6-benzyl-5-chloro[1,2,4]triazolo[1,5-a]pyrimidin-7(3H)-one | C12 H9 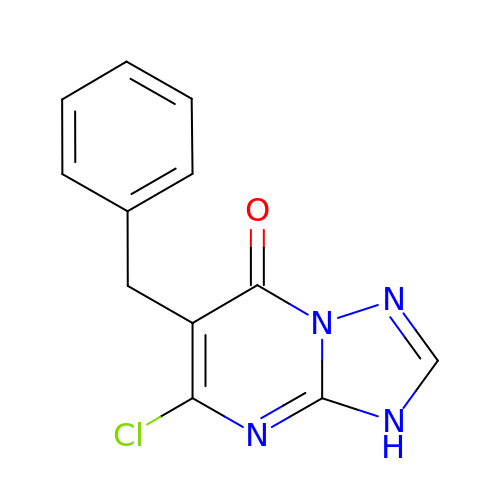Cl N4 O | MQEBPOLOTAZMKF-UHFFFAOYSA-N>[2x]TTNKPIVLSTWNFGLHANVEAWKVLSKGGKALDAVEKGVRLVEDDPTERSVGYGGR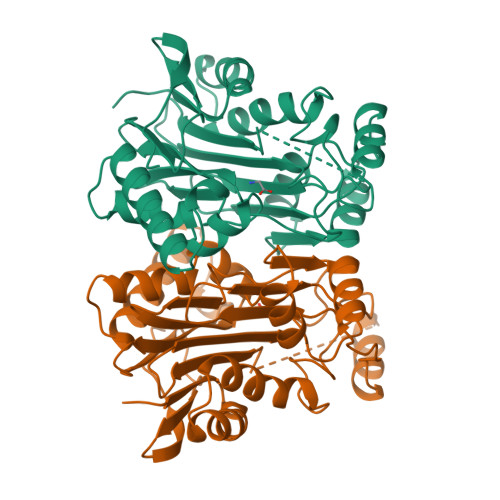PDRDGRVTLDACIMDENYNIGSVACMEHIKNPISVARAVMEKTPHVMLVGDGALEFALSQGFKKENLLTAESEKEWKEWLKTSQYKPIVNIENHDCIGMIALDAQGNLSGACTTSGMAYKMHGRVGDSPIIGAGLFVDNEIGAATATGHGEEVIRTVGTHLVVELMNQGRTPQQACKEAVERIVKIVNRRGKNLKDIQVGFIALNKKGEYGAYCIQDGFNFAVHDQKGNRLETPGFALK>MSLQRIVRVSLEHPTSAVCVAGVETLVDIYGSVPEGTEMFEVYGTPGVDIYISPNMERGRERADTRRWRFDATLEIIVVMNSPSNDLNDSHVQISYHSSHEPLPLAYAVLYLTCVDISLDCDLNCEGRQDRNFVDKRQWVWGPSGYGGILLVNCDRDDPSCDVQDNCDQHVHCLQDLEDMSVMVLRTQGPAALFDDHKLVLHTSSYDAKRAQVFHICGPEDVCEAYRHVLGQDKVSYEVPRLHGDEERFFVEGLSFPDAGFTGLISFHVTLLDDSNEDFSASPIFTDTVVFRVAPWIMTPSTLPPLEVYVCRVRNNTCFVDAVAELARKAGCKLTICPQAENRNDRWIQDEMELGYVQAPHKTLPVVFDSPRNGELQDFPYKRILGPDFGYVTREPRDRSVSGLDSFGNLEVSPPVVANGKEYPLGRILIGGNLPGSSGRRVTQVVRDFLHAQKVQPPVELFVDWLAVGHVDEFLSFVPAPDGKGFRMLLASPGACFKLFQEKQKCGHGRALLFQGVVDDEQVKTISINQVLSNKDLINYNKFVQSCIDWNREVLKRELGLAECDIIDIPQLFKTERKKATAFFPDLVNMLVLGKHLGIPKPFGPIINGCCCLEEKVRSLLEPLGLHCTFIDDFTPYHMLHGEVHAGTNVCRKPFSFKWWNMVP[2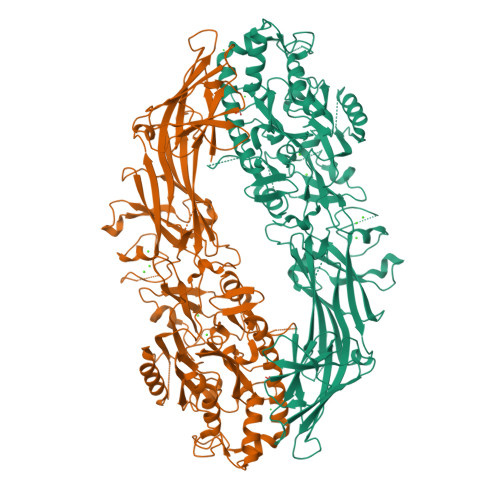x]>SDLWVQKMKTYFNRIDFDKDGAITRMDFESMAERFAKESEMKAEHAKVLMDSLTGVWDNFLTAVAGGKGIDETTFINSMKEMVKNPEAKSVVEGPLPLFFRAVDTNEDNNISRD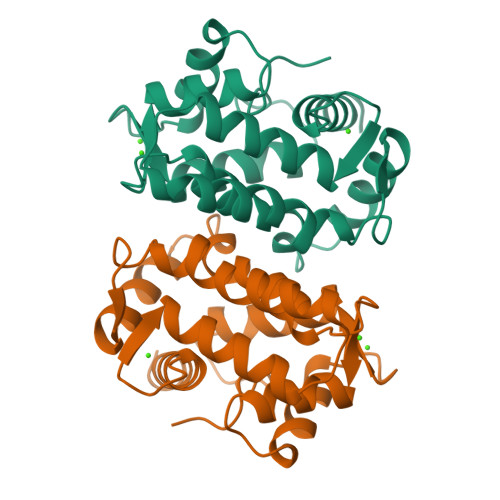EYGIFFGMLGLDKTMAPASFDAIDTNNDGLLSLEEFVIAGSDFFMNDGDSTNKVFWGPLV[2x]9-CYCLOPENTYL-6-{2-[3-(4-METHYL-PIPERAZIN-1-YL)-PROPOXY]-PHENYLAMINO}-9H-PURINE-2-CARBONITRILE | C25 H32 N8 O | 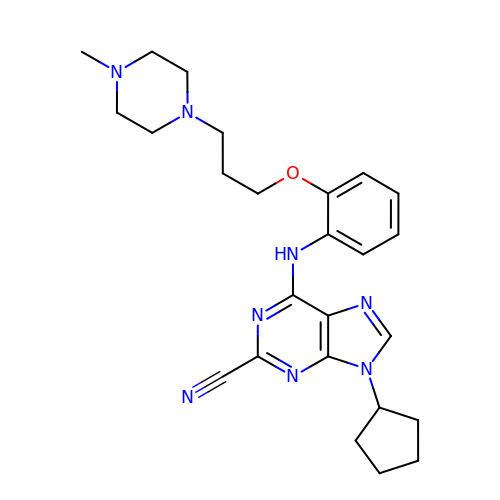VWGLHPDSAYQVRM-UHFFFAOYSA-N>[2x]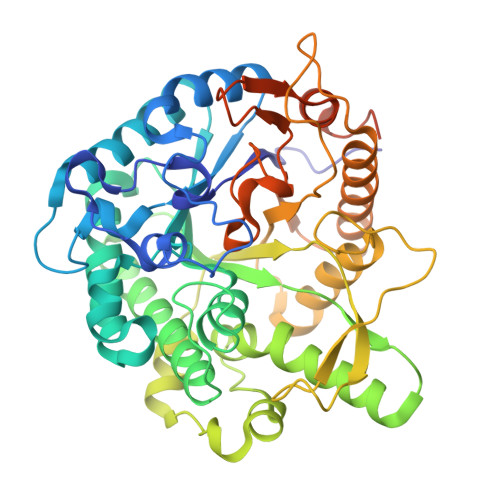MIKFPDQFLWGAATSAYQIEGSPLADGAGPSIWHRFVHSPGLTAKGETGDIACDHYNRYRDDIALMRSLGLQAYRFSVNWGRIFPDGTGRLNSAGLDFYERLVDALLEAGIEPLATLYHWDLPAALDDRGGWLNPEIAHWFADYAGAMFERLDGRVKRWATLNEPWVITDGGYLHGALAPGHRNVFEAPIASRNLMLAHGAAVQRYRQAGKHEIGLVVNIEPKYPASESDSDRNAAARSDAYMNRQYLDPAFGLGCPTEMAEIFGPAWRDWTAEELALAAQPIDWLGINYYTRGVMKHDDAKPPVRADYVRQPGATYTETGWEVFEQGLTETLLWVKERYGDIPLYVTENGSAFDDPPTAQGGRLEDPARVDYLERHLRAVHAAIAGGADVRGYMAWSLLDNLEWSLGFSKRFGIVHIDFETQQRTPKDSARLYSTVIASNGAVLSESAGAAPRAEPGIASAAEKLAAALEHHHHHH> MRSVISEQSLASTKTQKLFNNLISKGQSKIPLLEGQLDEESLTKTWGAFGLYLSRQLRMGRGTNIPHFGTFTFSAPECNLTGVTNPIERDKQFRVPVFLVSKEFVLGQPIKTGIFIDKHIRPYNVQTSGSISVTKINFTEIAQYADQNKEAVKISFERIIRQLADQTRQKRVVDMEIPGIGVFQVRNNIAAVHFDEYLIQNIKGVPKRPLSERKQKGDMNLTADRLSMLENTSRIGADAEQYLKTKLGIDIDNISTKSRPLTAVRNASTSNLLQPNNKTLQRPATSTTLRQSAINLKQPELGPLEFGLKRLKFWIRQNCFNAQDAFLEMCNCALGRTRAQRVKVDYKQFFEAINKMELDLNEEQIQELFKQLDANKDGYINYTDWRNTIKDDNDHLQYIKDVIYKRQLHTDDVLKTMGLDREHPPINKYQLKDALKKLDLTLTDIKAIRVAQTLLGHEEYISMYDLARSFETIEEDDKIFDPSWFKDILYKIKQKIMALENPNEIRESFENYDEHNEGILDTANFKTCLMRSQLKLTVKEINRIVRYLPKVKVNNIDYYNFLKLVERVDINASAPDAVSDISEFAVKLGKFIKDKKFTIPSFLKTVRRFSFVLDSSNNQDYFVTLTQMSEFLHRNVFKGNDRLDIDFYVNELDIDCDGYIKENDVQSFLNRYTYFDQ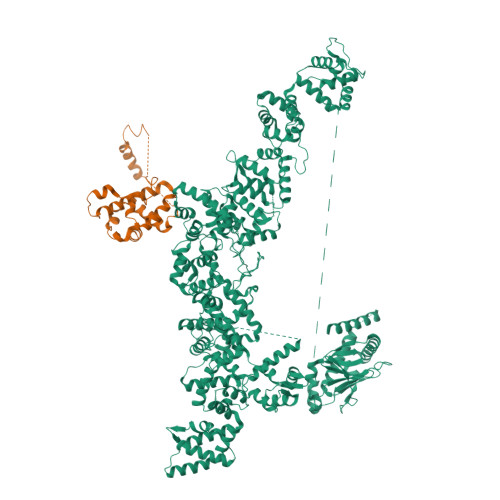TQYTPLSMTRSLTLKSLDPRTVSMNTKTLYPFKALSEAKVDTILRDLRKKMELKKMKAAELFSTLDADQDGFLTINEFSENIRKIIELSQPAIDGFFAYMDKLHTGMVDLSSFLKVMRKSIVTKDQPIKEDNFDWENEMVFRIRQWFKKEGITVEDSFRAIDQNFKREINVDDLEIFLKDCLKVKSEELNKAKLDRLFKLIDQYKRGKVNFVDWKRFIMEDFGYGMNQTIMGGKKIDNISSFDWKINARQQLGLVLTRRFSTLSHSFDVISGYRKKLLFSHFKKWVQDTDALRGFDLTESLMQELFSDLDSHNKGYLSESDWEIAFGGFDWEHQMHEEIKEYVKQNFKSIEKAFEFFCQGNQNKIIEQADFNKAINSILPKRFIDSDLKDLWVYVSSGQPQVDFHRFKIAFQKYIPHYERTIEYDQENMRPKTAGPLSSLSKSTSWNNIYGASQLNGNSQNPFGTSSIVDGNEDDVFEEKLLSKIRRLLRPTIKSVKKVLEQLDVNNIGYITNLEFRNAIKTLNLGLAQNEVDLLLNICEIDGRVNIKQFLKFIDFSESDKKIVQRSILKLREITNQVYTFLLSPKDAFRMFDVDSNGYLDFDQFSQFIGKLSQLSGHDMLPYSIIKDLFEYIDSKKDGVIDQAEWMDIFNKFEYVPQASINKQPLSKATVYNLQKRPQTSFNKSTLNELPHNKFNLEYISSNYPLTVKNEKIHQISDKEKYGTMNKFFDEVERQPESKPVQDNHFNQILGEWGKTKEFDKIIISIGKNRRFLLDMFGSLQQRNIPITFERAKAIIGQMLRNSGQSLKEESWPIILKFAERNGLIDYKFLLEVYKERIKRIDSHPIMSRNRSLQKFTS;> MQSTITSTTSLTPQQILNQIIKPEYIKYYSDWIHTANEKEARGLQLLGAIYKHKGSKKFRAKPPSVQLQQLHAQQEFDFQKAEEMYRKSQITSSYGQEFGYLQKDLKPTQNVFKYKKCSDLPFAKPLSDLAKLFIDNWIELNDELEFQELVLACLRSLHSRCIAQEVPKTEMKTKYEWKEDWNLSKPIRIDKAGSDLKAYKTNYNAIFKQRLKQEHINEQLKQLDNSDFAKQLKIFKPFKIN> MHHHHHHSSGRENLYFQGQLKNLPFYDVLDVLIKPTSLVQSSIQRFQEKFFIFALTPQQVREICISRDFLPGGRRDYTVQVQLRLCLAETSCPQEDNYPNSLCIKVNGKLFPLPGYAPPPKNGIEQKRPGRPL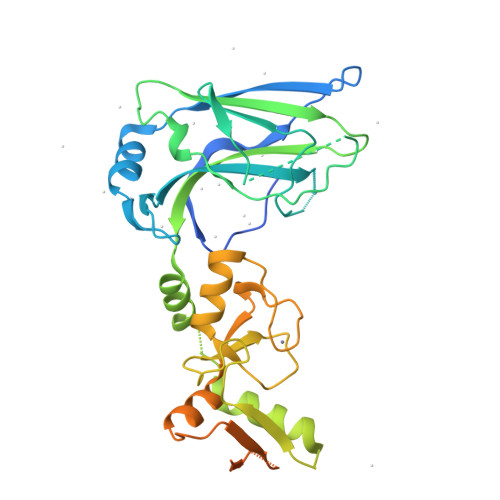NITSLVRLSSAVPNQISISWASEIGKNYSMSVYLVRQLTSAMLLQRLKMKGIRNPDHSRALIKEKLTADPDSEIATTSLRVSLMCPLGKMRLTIPCRAVTCTHLQCFDAALYLQMNEKKPTWICPVCDKKAAYESLILDGLFMEILNDCSDVDEIKFQEDGSWCPMRPKKEAMKVSSQPCTKIESSSVLSKPCSVTVASEASKKKVDVIDLTIESSSDEEEDPPAKR>[2x]MIKLCREVWIEVNLDAVKKNLRAIRRHIPHKSKIMAVVKANGYGHGSIEVARHALEHGASELAVASVEEGIVLRKAGITAPILVLGFTSLSCVKKSAAWNITLSAFQVDWMKEANEILEKEASANRLAIHINVDTGMGRLGVRTKEELLEVVKALKASKFLRWTGIFTHFSTADEPDTTLTKLQHEKF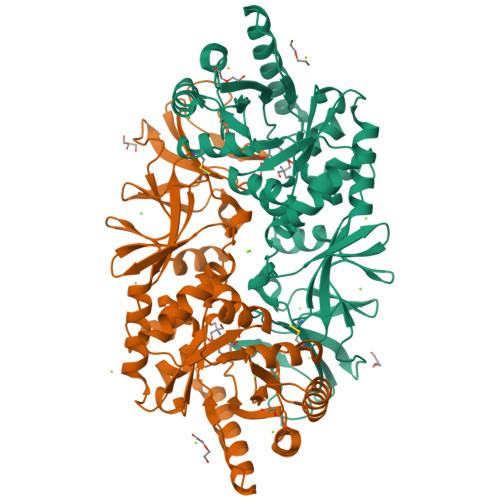ISFLSFLKKQGIELPTVHMCNTAAAIAFPEFSADMIRLGIGLYGLYPSAYIKQLNLVKLEPALSLKARIAYVKTMRTEPRTVSYGATYIAEPNEVIATLPIGYADGYSRALSNRGFVLHRGKRVPVAGRVTMDMIMVSLGENGEGKQGDEVVIYGKQKGAEISVDEVAEMLNTINYEVVSTLSRRIPRFYIRDGEIFKVSTPVLYV> DMRPEIR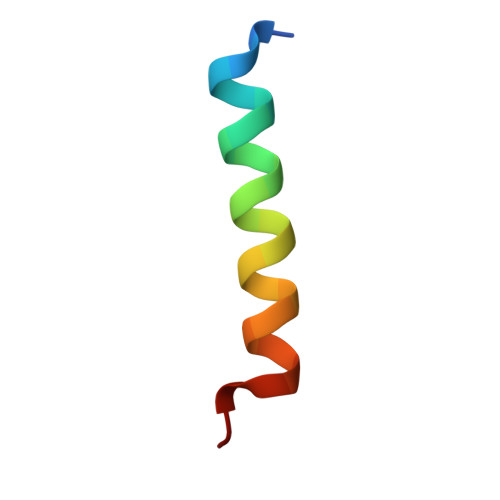IAQELRRIGDEFNATYARR N,N-dimethyl-5-(piperidin-4-yl)-1,2,4-oxadiazol-3-amine | C9 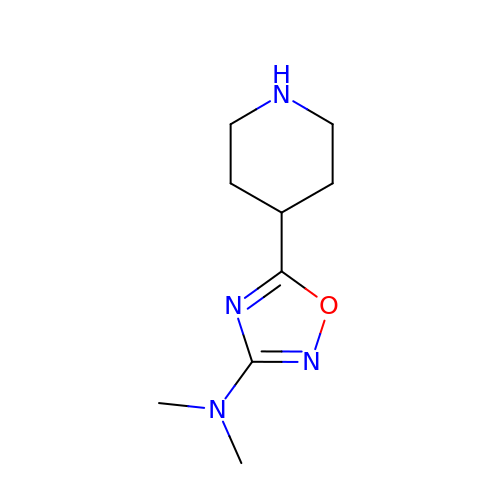H16 N4 O | STXBTTYNIARXAD-UHFFFAOYSA-N>PVQGSHVEGGVVEHPDAKDFGSAAALPADPTWFKHAVFYEVLVRAFFDASADGSGDLRGLIDRLDYLQWLGIDCIWLPPFYDSPLRDGGYDIRDFYKVLPEFGTVDDFVALVDAAHRRGIRIITDLVMNHTSESHPWFQESRRDPDGPYGDYYVWSDTSERYTDARIIFVDTEESNWSFDPVRRQFYWHRFFSHQPDLNYDNPAVQEAMIDVIRFWLGLGIDGFRLAAVPYLFEREGTNCENLPETHAFLKRVRKVVDDEFPGRVLLAEANQWPGDVVEYFGDPNTGGDECHMAFHFPLMPRIFMAVRRESRFPISEIIAQTPPIPDMAQWGIFLRNHDELTLEMVTDEERDYMYAEYAKDPRMKANVGIRRRLAPLLDNDRNQIELFTALLLSLPGSPVLYYGDEIGMGDVIWLGDRDGVRIPMQWTPDRNAGFSTANPGRLYLPPSQDPVYGYQAVNVEAQRDTSTSLLNFTRTMLAVRRRHPAFAVGAFQELGGSNPSVLAYVRQVAGDDGDTVLCVNNLSRFPQPIELDLQQWTNYTPVELTGHVEFPRIGQVPYLLTLPGHGFYWFQLTT[4x]

Mtb persister formation is dependent on the trehalose catalytic shift, a stress-responsive metabolic remodeling mechanism in which the disaccharide trehalose is liberated from cell surface glycolipids and repurposed as an internal carbon source to meet energy and redox demands. Here, using a biofilm-persister model, metabolomics, and cryo-electron microscopy (EM), we found that azidodeoxy- and aminodeoxy-d-trehalose analogues block the Mtb trehalose catalytic shift through inhibition of trehalose synthase TreS (Rv0126), which catalyzes the isomerization of trehalose to maltose. Specifically, TreS-catalyzed isomerization of recycled trehalose into maltose is a key step in the trehalose catalytic shift that promotes Mtb survival during stress. Although TreS is not strictly essential for Mtb viability under favorable growth conditions, it is required for the formation of biofilm persisters and can therefore, in principle, be conditionally targeted as a persistence factor.

Previously published results using Msmeg TreS unambiguously identified the aspartic acid residue corresponding to the D238 residue of Mtb TreS as the nucleophile that initiates the attack on the anomeric carbon of either trehalose or maltose. Therefore, we constructed a catalytically inactive Mtb TreS-D238A variant, which was used to obtain a cryo-EM structure of Mtb TreS in complex with a trehalose analogue inhibitor. Following multiple rounds of manual and computational real space refinement, clear density corresponding to a disaccharide molecule was observed near the C-terminal end of the β-sheets of the barrel where the active site of a TIM-barrel fold protein is typically located.48 The observed density for 6-TreAz was stronger for the D chain of the tetramer compared to the other 3 chains. The 6-azido-glucosyl moiety of 6-TreAz fit within the cryo-EM map is modeled with multiple axial hydroxyls as that is the best fit. This higher-energy conformation may derive from steric hindrance between the C6 azido group and the enzyme active site residues, or it may reflect a conformational change in the substrate required to promote catalysis. The structural alignment of the published ligand-free TreS structure with the solved crystal structure of wild-type TreS protein incubated with 6-TreAz shows no structural differences. However, as shown in Figure 5C, the 6-TreAz-bound cryo-EM structure shows significant movement of the L19 and L20 loops at the active site along with the H9 and H10 helices and L8 loop vacating the space required to accommodate 6-TreAz binding. However, the E280 residue, which acts as the general acid, moves slightly away from the ligand binding site to better accommodate the ligand and afford the acid/base chemistry essential for the enzymatic reaction. Additionally, D350, which is essential for coordinating ligand binding, moves toward the substrate and forms a hydrogen-bonded interaction with each of the two rings of 6-TreAz.N-(1H-benzimidazol-2-yl)-3-(4-fluorophenyl)-1H-pyrazole-4-carboxamide | C17 H12 F N5 O | 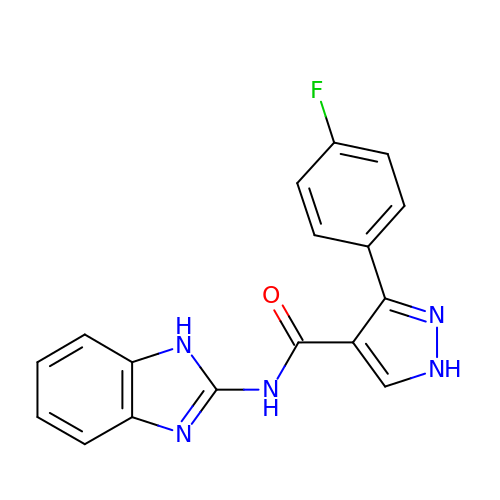NATFUWRFXYXTFK-UHFFFAOYSA-N> GPLGSGGGTIAMLNEISSDTLEQLYSLAFNQYQSGKYEDAHKVFQALCVLDHYDSRFFLGL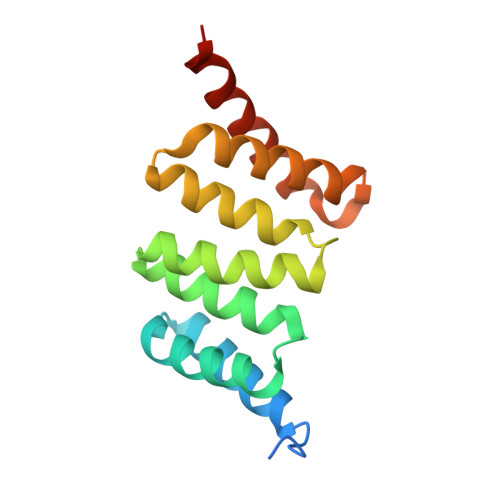GACRQAMGQYDLAIHSYSYGAVMDIKEPRFPFHAAECLLQKGELAEAESGLFLAQELIANKPEFKELSTRVSSMLEAIKLKKEMKHE>GMPNYKLTYFNMRGRAEIIRYIFAYLDIQYEDHRIEQADWPEIKSTLPFGKIPILEVDGLTLHQSLAIARYLTKNTDLAGNTEMEQCHVDAIVDTLDDFMSCFPWAEKKQDVKEQMFNELLTYNAPHLMQDLDTYLGGREWLIGNSVTWADFYWEICSTTLLVFKPDLLDNHPR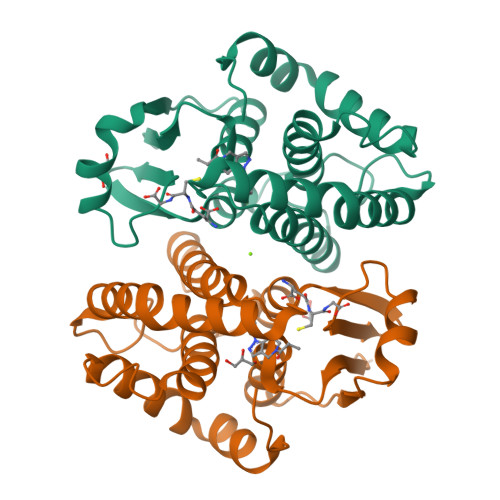LVTLRKKVQAIPAVANWIKRRPQTKL[2x]> GSGSGSGMSWIKEGELSLWERFCANIIKAGPMPKHIAFIMDGNRRYAKKCQVERQEGHSQGFNKLAETLRWCLNLGILEVTVYAFSIENFKRSKSEVDGLMDLARQKFSRLMEEKEKLQKHGVCIRVLGDLHLLPLDLQELIAQAVQATKNYNKCFLNVCFAYTSRHEISNAVREMAWGVEQGLLDPSDISESLLDKCLYTNRSPHPDILIRTSGEVRLSDFLLWQTSHSCLVFQPVLWPEYTFWNLFEAILQFQMNHSVLQKARDMYAEERKRQQLERDQATVTEQLLREGLQASGDAQLRRTRLHKLSARREERVQGFLQALELKRADWLARLGTASA;> GSGSGSGRGGSCLAAAHHRMRWRADGRSLEKLPVHMGLVITEVEQEPSFSDIASLVVWCMAVGISYISVYDHQGIFKRNNSRLMDEILKQQQELLGLDCSKDKDDQVLNCHLAVKVLSPEDGKADIVRAAQDFCQLVAQKQKRPTDLDVDTLASLLSSNGCPDPDLVLKFGPVDSTLGFLPWHIRLTEIVSLPSHLNISYEDFFSALRQYAACEQRLGK

The human cis-prenyltransferase (hcis-PT) complex catalyzes the formation of dehydrodolichyl diphosphate (DHDD, C85–100), a long-chain isoprenoid, by chain elongation of farnesyl diphosphate (FPP, C15) via multiple condensations with IPP. DHDD is the precursor for dolichol-phosphate, the lipidic glycosyl carrier crucial for N-linked protein glycosylation. Localized to the endoplasmic reticulum, hcis-PT is composed of two structurally and functionally distinct subunit types. These include the catalytically active DHDD synthase (DHDDS) and the quiescent Nogo-B receptor (NgBR) subunits.

Indeed, this construct (termed hereafter xcis-PT) resulted in well-diffracting crystals while demonstrating unperturbed catalytic activity, allowing us to determine its structure in complex with Mg2+ and FPP at 2.3 Å resolution. The asymmetric unit (ASU) contains a single heterodimer, with Mg2+–FPP and an additional phosphate moiety bound only at the DHDDS active-site. Moreover, it reveals the structural organization of the DHDDS C-terminal domain, exhibiting a “helix-turn-helix” motif fold not observed in other cis-prenyltransferases, which facilitates complex tetramerization via a dimer-of-heterodimers assembly mode. Importantly, this tetramer is formed by both homotypic interactions between DHDDS “helix-turn-helix” motifs and heterotypic interactions of the “turn” region with sNgBR from adjacent ASUs, burying a total surface area of 793.3 Å2. The active-site contains two substrate-binding sites: an S1 site, which binds the initiatory substrate FPP, and an S2 site, which binds the IPP molecules used for chain elongation, and is occupied by the phosphate molecule in our structure. At the S1 site, the pyrophosphate moiety of FPP interacts with a Mg2+ ion. This Mg2+ ion, which plays a crucial role in pyrophosphate hydrolysis during the condensation reaction, is octahedrally coordinated by two of the pyrophosphate oxygens, three surrounding water molecules, and one carboxylate oxygen of the strictly conserved D34. In addition to the interaction with the Mg2+ ion, the pyrophosphate moiety is also directly stabilized by R37 and R38 from helix α1, and R85 from the βB–α3 linker. While xcis-PT was crystallized in the absence of IPP, a phosphate molecule occupying the IPP pyrophosphate group position, as observed in other cis-prenyltransferases, is present at the S2 site and is stabilized through a concerted coordination by the conserved R205, R211, and S213. Specifically, strands βΑ, βΒ, and βD and helices α1 and α6 are tightly packed via hydrophobic interactions, leaving this region without a detectable substrate-binding cavity and completely devoid of water molecules.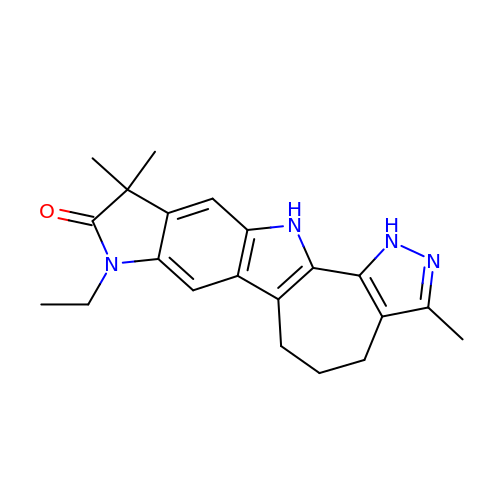8-ethyl-3,10,10-trimethyl-4,5,6,8,10,12-hexahydropyrazolo[4',3':6,7]cyclohepta[1,2-b]pyrrolo[2,3-f]indol-9(1H)-one | C21 H24 N4 O | AOMMPEGZDRAGRC-UHFFFAOYSA-N>[2x]QVGS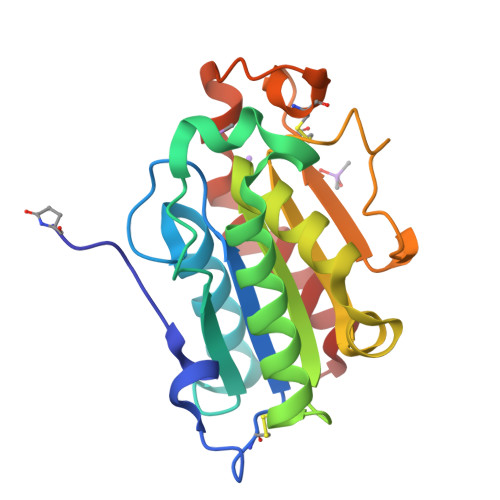SKNELETGSASNCPKAILIFARGSTETGNLGTLGAPLGDALESRYGASNVWVQGVGGPYDAALGDNALPRGSSAAAIREGVRLLNLANSKCPNSKVVAGGYSQGAALAAAAISDASTTVRNQIVGTVLFGYTKNQQNRGGIPGYPQDRLRVYCAVGDLVCEGTLIVLAPHLSYGDEARNEAPAFLISKIGN>GPHMEELRERVWNGTINVEVVVSDAIVVPNTTLADKSCHIVMLRDAYLGFYLPTVVRKLADTIKVPYESDYRNWWFEYNGEGVPWEYP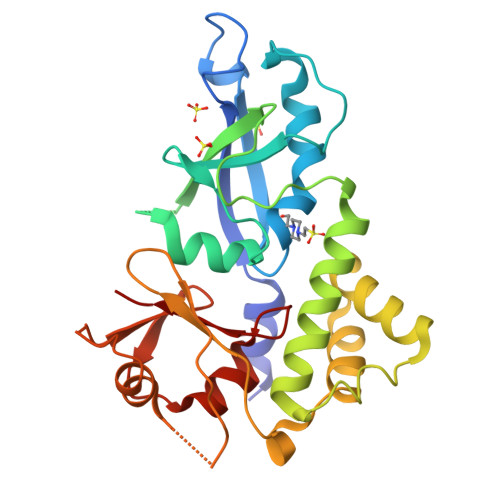CGVLFDLLNKKRKKQGNELDDTSLQMWELQLCHGDKYPRGILPLVDGHSQIKDYWRHQWKQACFILNGSAKRIMSLSIPDFENFWVSILSRNRSDFMAVRSKLFSMNKAKSLPVRVWTSNYAVLQPTVPVTDKELSVAELLDSIKLSSDGVKSVIIQGIDVSIEDNIFELYDIFASIDGFLYLVTK[5x]>[2x]GPNCAPGQKVKLFRASEPILSVLMWGVNHTINELSNVPVPVMLMPDDFKAYSKIKVDNHLFNKENLPSRFKFKEYCPMVFRNLRERFGIDDQDYQNSVTRSAPINSDSQGRCGTRFLTTYDRRFVIKTVSSEDVAEMHNILKKYHQFIVECHGNTLLPQFLGMYRLTVDGVETYMVVTRNVF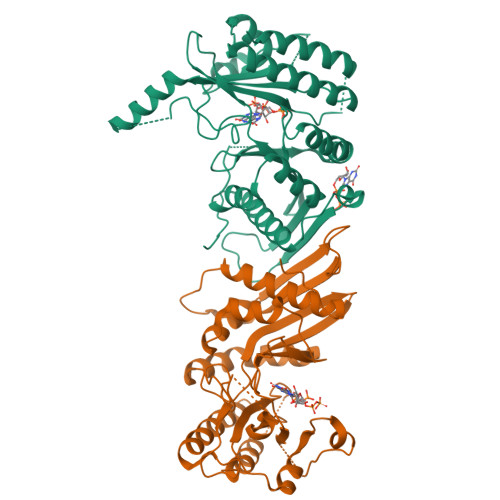SHRLTVHRKYDLKGSTVAREASDKEKAKDLPTFKDNDFLNEGQKLHVGEESKKNFLEKLKRDVEFLAQLKIMDYSLLVGIHDVDRAEQEEMEVEERAEDEECENDGVGGNLLCSYGTPPDSPGNLLSFPRFFGPGEFDPSVDVYAMKSHESSPKKEVYFMAIIDILTPYDTKKKAAHAAKTVKHGAGAEISTVNPEQYSKRFNEFMSNILT>YLSIAFPENTKLDWKPVTKNTRYCPMGGEWFLEPGLQEESFLSSTPIGATPSKSDGFLCHAAKWVTTCDFRWYGPKYITHSIHNIKPTRSDCDTALASYKSGTLVSLGFPPESCGYASVTDSEFLVIMITPHHVGVDDYRGHWVDPLFVGGECDQSYCDTIHNSSVWIPADQTKKNICGQSFTPLTVTVAYDKTKEIAAGGIVFKSKYHSHMEGARTCRLSYCGRNGIKFPNGEWVSLDVKTRIQEKHLLPLFKECPAGTEVRSTLQSDGAQVLTSEIQRILDYSLCQNTWDKVERKEPLSPLDLSYLASKSPGKGLAYTVINGTLSFAHTRYVRMWIDGPVLKEPKGKRESPSGISSDIWTQW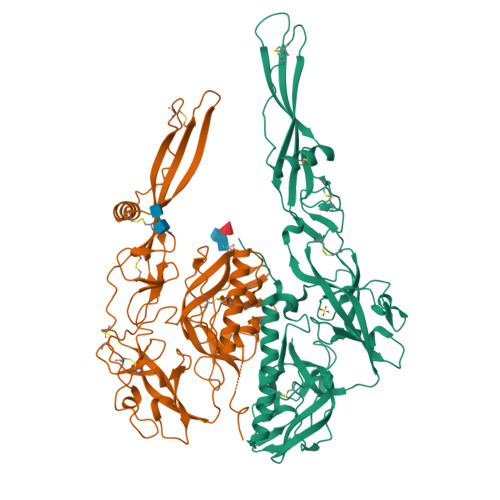FKYGDMEIGPNGLLKTAGGYKFPWHLIGMGIVDNELHELSEANPLDHPQLPHAQS[4x]> VNQQLNSATKLFSVKLGATRVIYHAGTAGATLSVSNPQNYPILVQSSVKAADKSSPAPFLVMPPLFRLEANQQSQLRIVRTGGDMPTDRETLQWVCIKAVPPENEPSDTQAKGATLDLNLSINACDK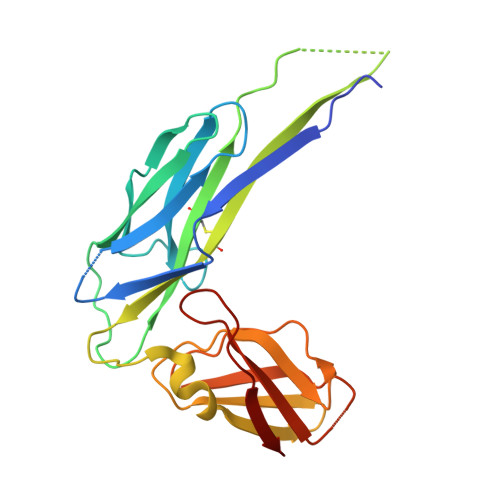LIFRPDAVKGTPEDVAGNLRWVETGNKLKVENPTPFYMNLASVTVGGKPITGLEYVPPFADKTLNMPGSAHGDIEWRVITDFGGESHPFHYVLK> GSHSKQALSEIETRHSEIIKLENSIRELHDMFMDMAMLVESQG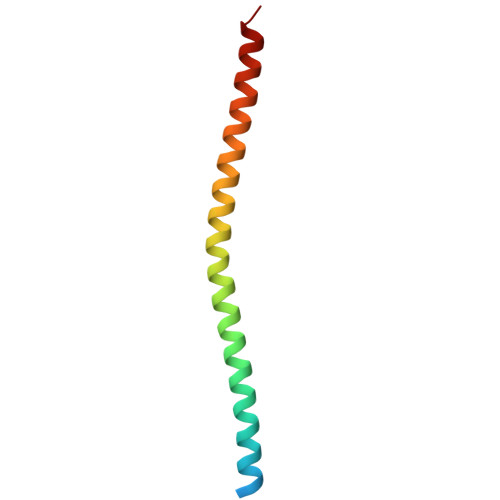EMIDRIEYNVEHAVDYVERAVSDTKKAVKYQS>[2x]KVDNMKVSVYGAGNQNLYINKLNLPEKFGGEPPYGGSRMAIEFAEAGHDVVLAEPNKNIMSDDLWKKVEDAGVKVVSDDVEAAKHGEIHVLFTPFGKATFRIAKTIIEHVPENAVICNTCTVSPVVLYYSLEPILRTKRKDVGISSMHPAAVPGTP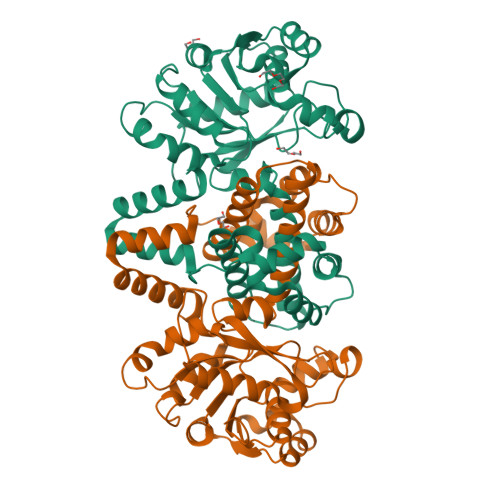QHGHYVIGGKTTDGKELATEEQIKKAVELAKSAGKEAYVVPADVSSVVADMGSLVTAVALSGVLDYYTVGRKIINAPKKMIEQQVIMTLQTMASLVETSGIEGMVKALNPELLIRSASSMKLLDRQKDLDAALEILQNLDETLKAEVEKAEIKPTTLVAAQSLVKEIKTLIGGAAAEGAIKRSARKLFEH> PNFSGNWKIIRSENFEELLKVLGVNVMLRKIAVAAASKE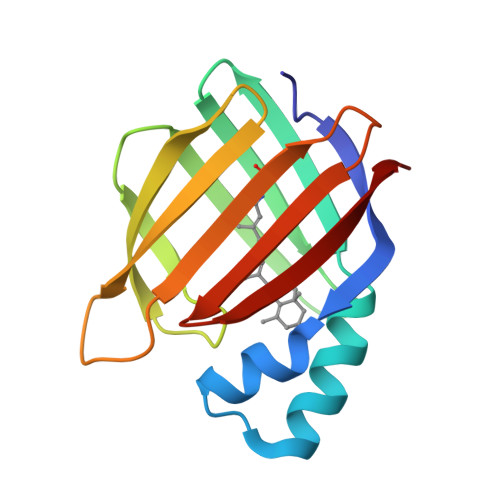AVEIKQEGDTFYIKVSTTVYTTEINFKVGEEFEEQTVDGRPCKSLVKWESENKMVCEQKLLKGEGPKTSWTKELTNDGELIETMTADDVVCTQVFVRE> MTLRSVCVFCGASPGASPVYQEAAVALGRHLAERGLTLVYGGGAVGLMGTVADAALAAGGEVIGIIPQSLQEAEIGHKGLTRLEVVDGMHARKARMAELADAFIALPGGLGTLEALFEVWTWGQLGYHAKPLGLLEVNGFYDPLLTFLD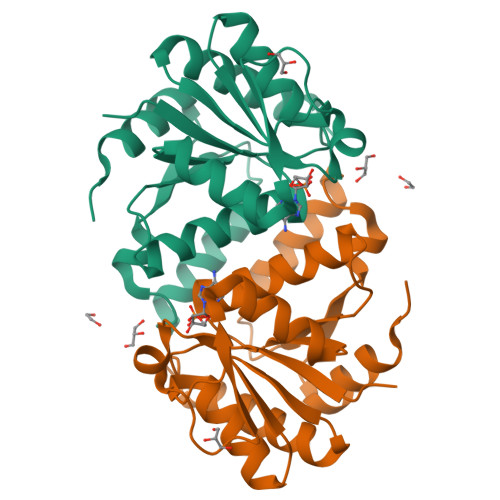HLVDERFVRAEHRGMLQRGASPEALLDALAAWTPSVAPKWVDRTPQLEHHHHHH>GSHMPNYKLLYFNMRGRAEIIRYIFAYLDIKYEDHRIEQADWPKIKPTLPFGKIPVLEVEGLTLHQSLAIARYLTKNTDLAGKTELEQCQVDAVVDTLDDFMSLFPWAEENQDLKERTFNDLLTRQAPHL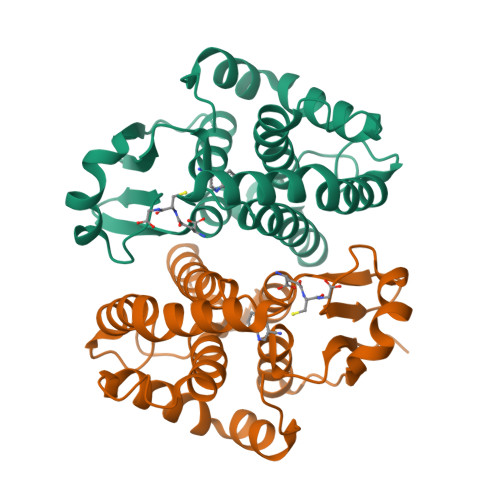LKDLDTYLGDKEWFIGNYVTWADFYWDICSTTLLVLKPDLLGIYPRLVSLRNKVQAIPAISAWILKRPQTKL[2x]>AK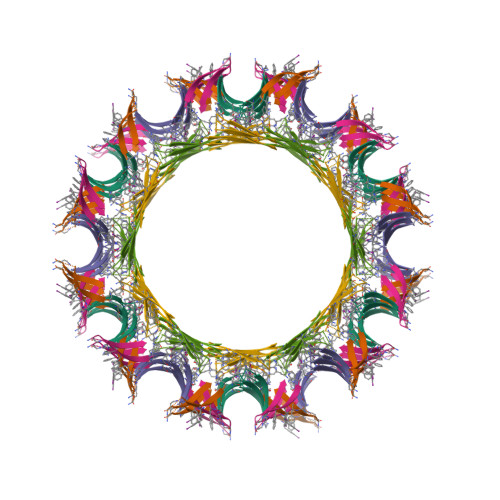LVFFAEAEAFFVLK[6x]>MTIPTLYMNDGMNAQSSQALHIQTYCNSVRQQIPVDFGRFPNLRESERQINTGLGAARQHAEHYLKDIQPLIIRNVTNIQDYFETQNLISTVMPSGATKEQWLSALGMVSDKAKEYQEVSANTRRTIGSLNDKLIIDSNNYQLIVVNLNNVVNGNNGVLEQLNRDIDGINAAIDGAIAGIVVGGLLVIGGAIVTAIGAVAGLVTAGTSTPVVMGGIAMMTAGAGGVIGGAIVLDKSLSAREKLYRDRSQLNSEVLVASQIGSGYRGLQTQAQSAVTAATQMNNAWDSLTSELETLNANLRKGIIDDSFLRQLFLTASQTSVTKVLDGTKIIKQQMAGVVVREVPANQSIADFVKRLAALEHHHHHH[10x]

Tripartite α-PFTs are members of the ClyA α-PFT family. Proteins in this family undergo a large scale conformational change from a compact soluble structure, where the hydrophobic residues are hidden often within a β-tongue motif, to an extended pore structure with the hydrophobic residues exposed in two extended α-helices which insert into the cell membrane. Here we show that S. marcescens has a tripartite haemolytic α-PFT (SmhABC), and propose a mechanism of pore assembly. We present the structures of the soluble A component (SmhA), as well as the soluble and pore conformations of the B component (SmhB).

Like the AhlB pore, the SmhB pore contained ten monomers of SmhB in two conformations (type 1 and type 2) which assemble into a ring with pseudo tenfold symmetry. Although the resolution of this structure was low, the electron density was clear and continuous for the protein chain, enabling a model to be built with residues truncated at Cβ. In addition, clear positive difference density could be observed in omit maps calculated with sections of the model deleted (residues 157–251 in chain A and B), indicating that the structure solution was correct. As seen in AhlB, the head domain of SmhB undergoes a large scale conformational change transforming from the soluble to pore forms, with the β-tongue substructure refolding to form extended hydrophobic helices to α3 and α4. The transformation from a soluble β-tongue containing structure to an extended helical pore structure seen in SmhB and modelled in SmhA, occurs in a similar way for A. hydrophila AhlB7. In order for this conformational change to occur, the C-terminal loop and helix α7 must move to free the β-tongue to form the two extended trans-membrane helices in the pore conformation (α3-α4), with the N-terminal helix (α1) also moving from parallel to α7 to an end to end packing, resulting in a narrower more compact tail. As the overall structures of the soluble and pore forms of SmhB are almost identical to those of AhlB (RMSD Cα 0.64 Å and 0.46 Å, respectively),, not surprising given the high level of sequence identity (62%), we investigated if these structural similarities also conveyed functional similarities. Haemolytic assays, replacing the SmhB component of the SmhABC pore with AhlB in a 1:1:1 ratio showed that this chimeric pore had the same lytic activity as the SmhABC pore.> ATCDDGRTTANAACCILFPILDDIQENLFDGAQCGEEVHESLRLTFHDAIGFSPTLGGGGADGSIIAFDTIETNFPANAGIDEIVSAQKPFVAKHNISAG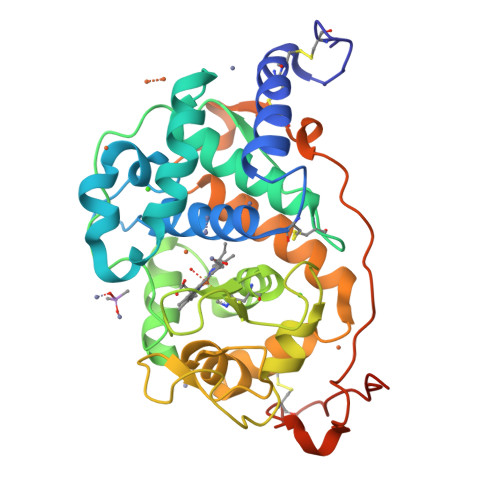DFIQFAGAVGVSNCPGGVRIPFFLGRPDAVAASPDHLVPEPFDSVDSILARMGDAGFSPVEVVSLLASHSIAAADKVDPSIPGTPFDSTPGVFDSQFFIETQLKGRLFPGTADNKGEAQSPLQGEIRLQSDHLLARDPQTACEWQSMVNNQPKIQNRFAATMSKMALLGQDKTKLIDCSDVIPTPPALVGAAHLPAGFSLSDVEQACAATPFPALTADPGPVTSVPPVPGS(2~{R},3~{S},4~{S},5~{R},6~{S})-2-(hydroxymethyl)-6-[(2~{R},3~{R},4~{S},5~{R},6~{S})-2-(hydroxymethyl)-6-[(2~{R},3~{R},4~{S},5~{R},6~{R})-2-(hydroxymethyl)-3,5-bis(oxidanyl)-6-[4-(thiophen-2-ylmethoxymethyl)-1,2,3-triazol-1-yl]oxan-4-yl]oxy-3,5-bis(oxidanyl)oxan-4-yl]oxy-oxane-3,4,5-triol 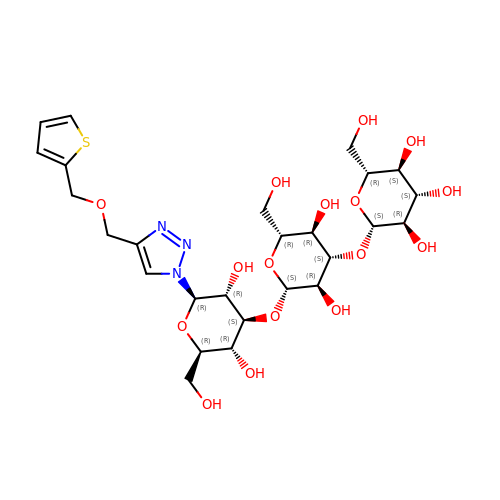| C26 H39 N3 O16 S | PCTXRGORDHBRNF-KACUVCQDSA-N(1S,3R,8AS)-8-(2-{(4S,6S)-3-(4-HYDROXY-3-METHOXYBENZYL)-4-[2-(METHYLAMINO)-2-OXOETHYL]-2-OXO-1,3-OXAZINAN-6-YL}ETHYL)-3,7-DIMETHYL-1,2,3,7,8,8A-HEXAHYDRONAPHTHALEN-1-YL (2R)-2-METHYLBUTANOATE | C34 H48 N2 O7 | 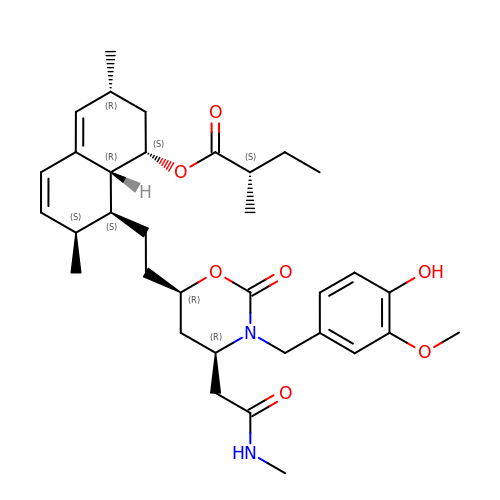XGCZRGJUCNQVCO-XFAJEYMZSA-N> MFGLIGHLTSLEQARDVSRRMGYDEYADQGLEFWSSAPPQIVDEITVTSATGKVIHGRYIESCFLPEMLAARRFKTATRKVLNAMSHAQKHGIDISALGGFTSIIFENFDLASLRQVRDTTLEFERFTTGNTHTAYVICRQVEAAAKTLGIDITQATVAVVGATGDIGSAVCRWLDLKLGVGDLILTARNQERLDNLQAELGRGKILPLEAALPEADFIVWVASMPQGVVIDPATLKQPCVLIDGGYPKNLGSKVQGEGIYVLNGGVVEHCFDIDWQIMSAAEMARPERQMFACFAEAMLLEFEGWHTNFSWGRNQITIEKMEAIGEASVRHGFQPLALAIENLYFQ;> MRTPWDPPNPTFSLSSVSGDRRLMPQLEASLELDFQSESYKDAYSRINAIVIEGEQEAFDNYNRLAEMLPDQRDELHKLAKMEQRHMKGFMACGKNLSVTPDMGFAQKFFERLHENFKAAAAEGKVVTCLLIQSLIIECFAIAAYNIYIPVADAFARKITEGVVRDEYLHRNFGEEWLKANFDASKAELEEANRQNLPLVWLMLNEVADDARELGMERESLVEDFMIAYGEALENIGFTTREIMRMSAY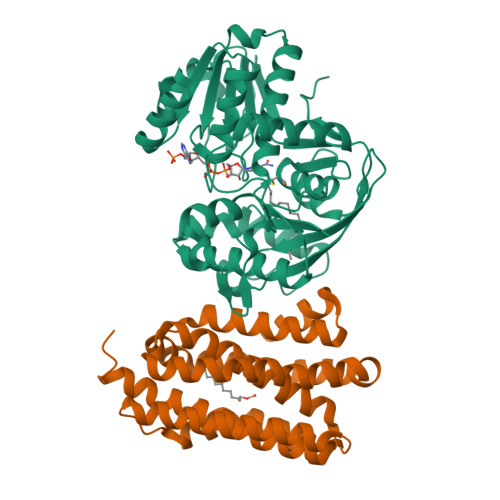GLAAV> ATRMAPVIMVPGSSASQNRFDSLITELGKETPKKHSVLKLTVQTDGTIKYSGSIAANDNEPFIVIGFANNRDGKANIDKQAVWLNTAFKALVKTYHFNHFYALGHSNGGLIWTLFLERYLKESPKVHIDRLMTIASPYNMESTSTTAKTSMFKELYRYRTGLPESLTVYSIAG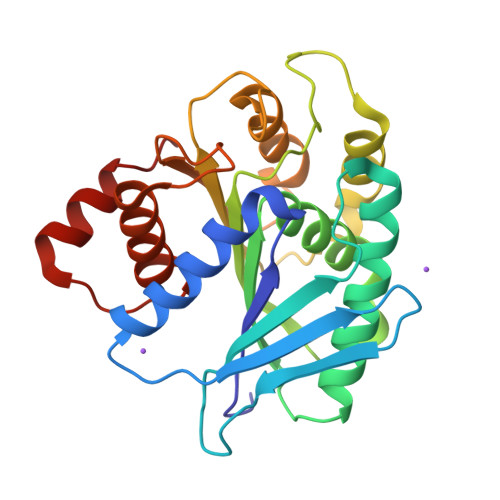TENYTSDGTVPYNSVNYGKYIFQDQVKHFTEITVTGANTAHSDLPQNKQIVSLIRQYLLAETMPDKVRQKNAQRVQN>MKETNFGEKTRVLVVGGTGSLGRRIVSACLAEGHETYVLQRPEIGVDIEKVQLLLSFKRLGAHLVEGSFSDHQSLVSAVKQVDVVVSAMSGVHFRTHNIPVQLKLVAAIKEAGNVKRFLPSEFGMDPSRMGHAMPPGSETFDQKMEIRNAIKAAGISHTYLVGACFAAYFGGNLSQMGTLFPPKNKVDIYGDGNVKVVFVDEDDMAKYTAKTLNDPRTLNKTVYVRPTDNILTQMELVQIWEKLTEKELEKTYVSGNDFLADIED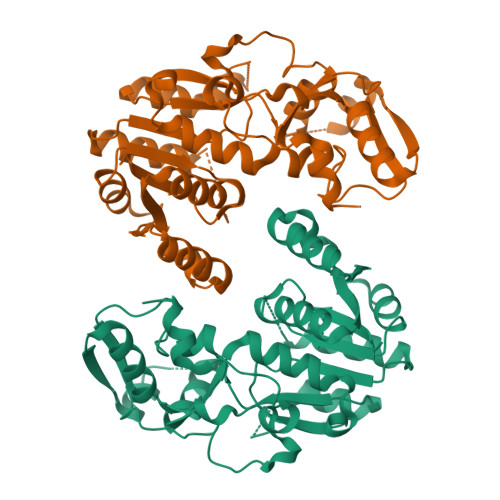KEISHQAGLGHFYHIYYEGCLTDHEVGDDEEATKLYPDVKYKRMDEYLKIFV[2x]>[2x]DRNSVDYAQIASGIDTRTTVMIKNIPNKFTQQMLRDYIDVTNKGTYDFLYLRIDFVNKCNVGYAFINFIEPQSIITFG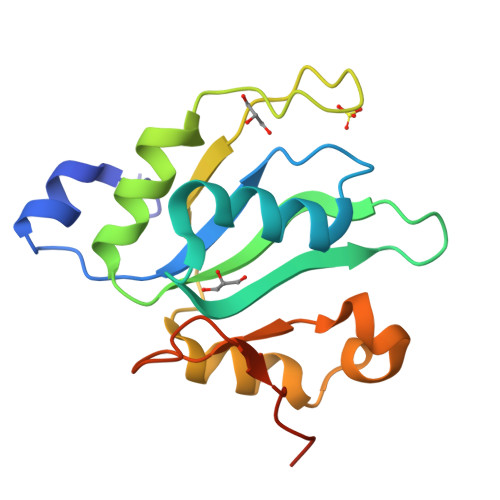KARVGTQWNVFHSEKICDISYANIQGKDRLIEKFRNSCVMDENPAYRPKIFVSHGPNRGMEEPFPAPNNARRKLRS(4~{S})-6-azanyl-4-[3-(2-fluorophenyl)-5-(trifluoromethyl)phenyl]-3-methyl-4-propan-2-yl-2~{H}-pyrano[2,3-c]pyrazole-5-carbonitrile 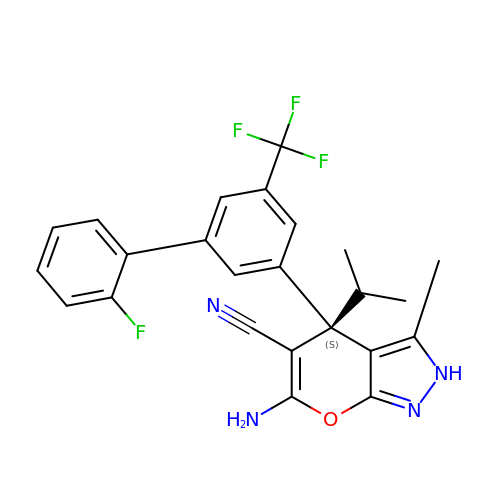| C24 H20 F4 N4 O | ODGVACPFBGBPRF-QHCPKHFHSA-N> NPCLTGPRTCKDLLDRGHFLSGWHTIYLPDCRPLTVLCDMDTDGGGWTVFQRRVDGSVDFYRDWATYKQGFGSRLGEFWLGNDNIHALTAQGTSELRTDLVDFEDNYQFAKYRSFKVADEAEKYNLVLGAFVEGSAGDSLTFHNNQSFSTKDQDNDLNTG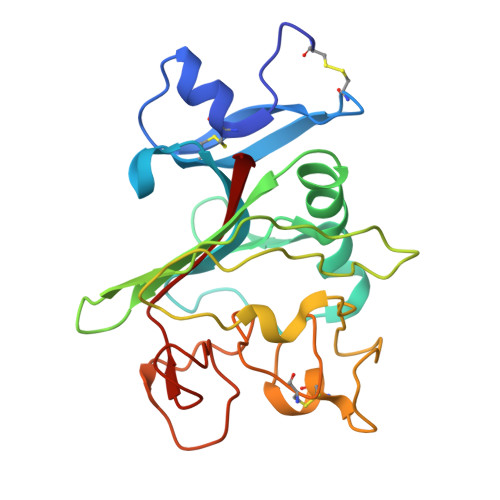NCAVMFQGAWWYKNCHTSNLNGRYLRGTHGSFANGINWKSGKGYNYSYKVSEMKVRPA>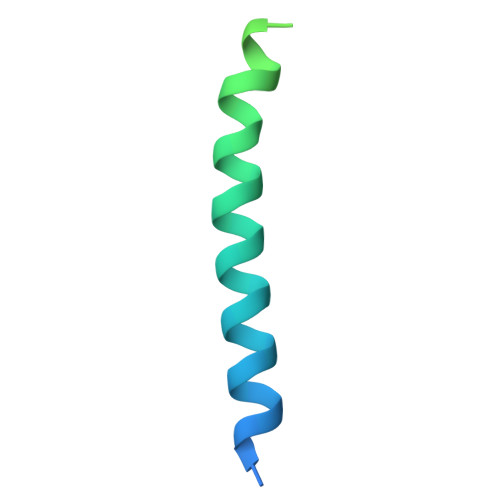 GPGSESSNISQESKLINTLTDENEKLREELQQYYALSDAKEEEPRYKALRGENQDLREKERKYQDKIKKLEEKEKNLEKKSED>NSVSMIGKIAETDVSGANFDGNNKLSFSLFFDEKIDASKGVPAIQILNENNELVKTIPLKDYNGQKGYINFEWDGTNEKGEKVPKGNYKIKAEYNLDSHSKQYLQTRIGRGEVES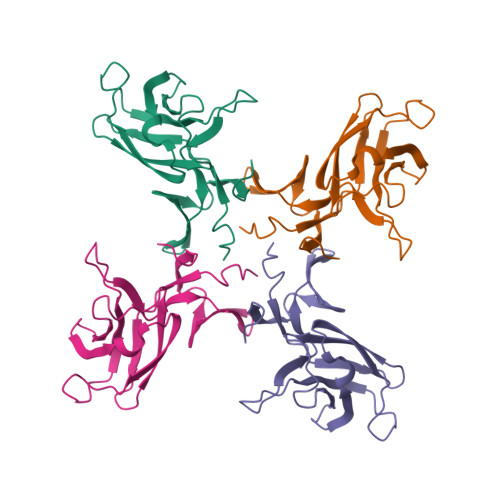VIFDKGKPMLRMGEMVLPIDSAIEFYQPDQK[4x]2,4-bis(fluoranyl)-6-(1~{H}-pyrazol-3-yl)phenol 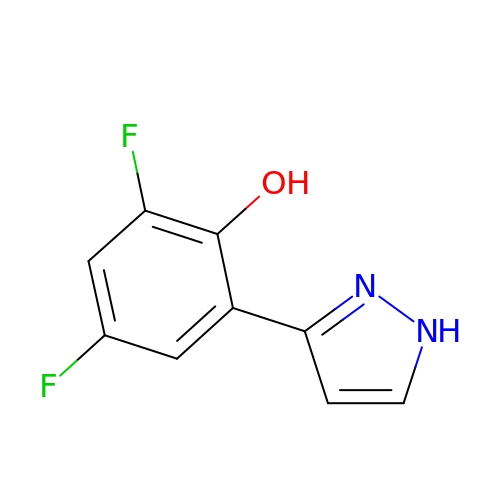| C9 H6 F2 N2 O | JUXBDWQXPZSIML-UHFFFAOYSA-N3-ISOBUTYL-1-METHYLXANTHINE | C10 H14 N4 O2 | 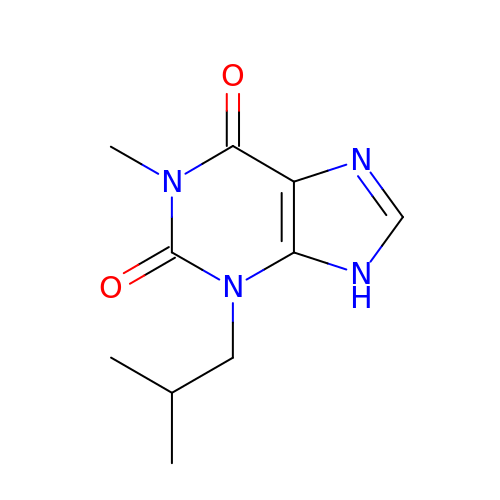APIXJSLKIYYUKG-UHFFFAOYSA-N> DKEEVQRKR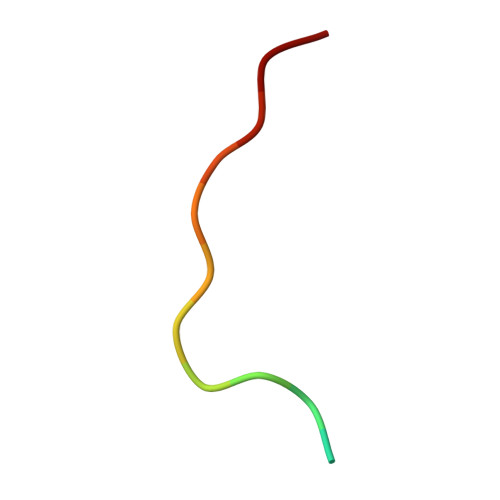QKLMP> GAMGYKDNIRHGVCWIYYPDGGSLVGEVNEDGEMTGEKIAYVYPDERTALYGKFIDGEMIEGKLATLMSTEEGRPHFELMPGNSVYHFDKSTSSCISTNALLPDPYESERVYVAESLISSAGEGLFSKVAVGPNTVMSFYNGVRITHQEVDSRDWALNGNTLSLDEETVIDVPEPYNHVSKYCASLGHKANHSFTPNCIYDMFVHPRFGPIKCIRTLRAVEADEELTV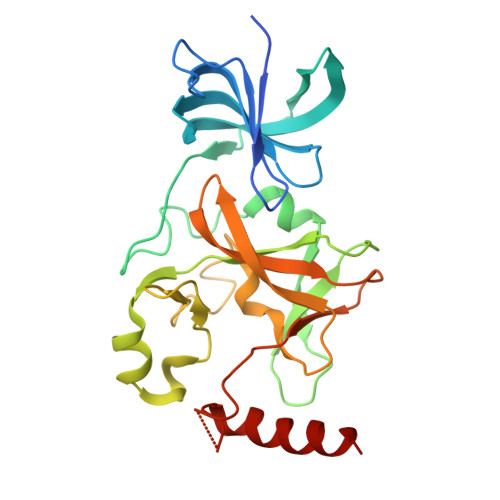AYGYDHSPPGKSGPEAPEWYQVELKAFQATQQK N-(tert-butoxycarbonyl)-L-alanyl-N-{(1R)-5-ammonio-1-[hydroxy(methoxy)boranyl]pentyl}-L-valinamide | C19 H40 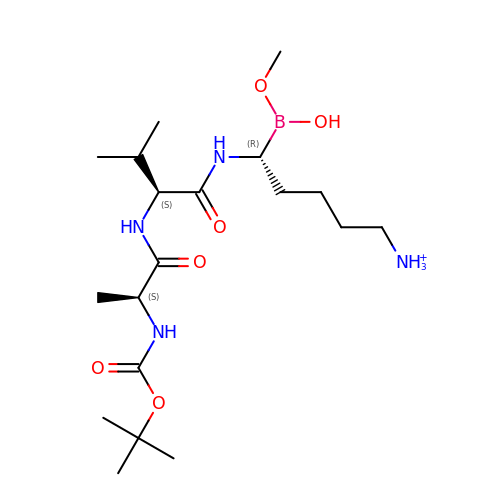B N4 O6 | OTTITSSTTJGNLR-KKUMJFAQSA-O> MTETIKCIGCGVEIQTEDKNEVGYAPASSLEKEQVICQRCFRLKHYNEIQDVSLTDDDFLRILNGIGKSDALVVKIVDIFDFNGSWLPGLHRFVGNNKVLLVGNKADLIPKSVKHDKVKHWMRYSAKQLGLKPEDVFL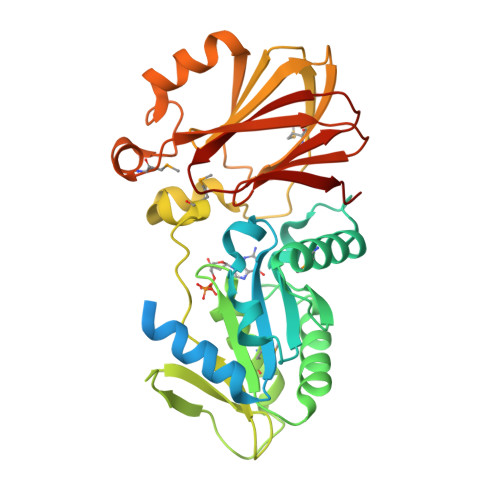ISAAKGQGIAELADAIEYYRGGKDVYVVGCTNVGKSTFINRMIKEFSDETENVITTSHFPGTTLDLIDIPLDEESSLYDTPGIINHHQMAHYVGKQSLKLITPTKEIKPMVFQLNEEQTLFFSGLARFDYVSGGRRAFTCHFSNRLTIHRTKLEKADELYKNHAGDLLSPPTPEELENMPELVKYEFNIREPKTDVVFSGLGWVTVNEPGAKIVAHVPKGVSVSLRKSLI>MTIKTKAELLNKWKPLLEGEGLPEIANSKQAIIAKIFENQEKDFQTAPEYKDEKIAQAFGSFLTEAEIGGDHGYNATNIAAGQTSGAVTQIGPAVMGMVRRAIPNLIAFDICGVQPMNSPTGQVFALRAVYGKDPVAAGAKEAFHPMYGPDAMFSGQGAAKKFPALAASTQTTVGDIYTHFFQETGTVYLQASVQVTIDAGATDAAKLDAEIKKQMEAGALVEIAEGMATSIAELQEGFNGSTDNPWNEMGFRIDKQVIEAKSRQLKAAYSIELAQDLRAVHGMDADAELSGILATEIMLEINREVVDWINYSAQVGKSGMTLTPGSKAGVFDFQDPIDIRGARWAGESFKALLFQIDKEAVEIARQTGRGEGNFIIASRNVVNVLASVDTGISYAAQGLATGFSTDTTKSVFAGVLGGKYRVYIDQYAKQDYFTVGYKGPNEMDAGIYYAPYVALTPLRGSDPKNFQPVMGFKTRYGIGINPFAESAAQAPASRIQSGMPSILNSLGKNAYFRRVYVKGI[186x];>[11x]MAKINELLRESTTTNSNSIGRPNLVALTRATTKLIYSDIVATQRTNQPVAAFYGIKYLNPDNEFTFKTGATYAGEAGYVDREQITELTEESKLTLNKGDLFKYNNIVYKVLEDTPFATIEESDLELALQIAIVLLKVRLFSDAASTSKFESSDSEIADARFQINKWQTAVKSRKLKTGITVELAQDLEANGFDAPNFLEDLLATEMADEINKDILQSLITVSKRYKVTGITDSGFIDLSYASAPEAGRSLYRMVCEMVSHIQKESTYTATFCVASARAAAILAASGWLKHKPEDDKYLSQNAYGFLANGLPLYCDTNSPLDYVIVGVVENIGEKEIVGSIFYAPYTEGLDLDDPEHVGAFKVVVDPESLQPSIGLLVRYALSANPYTVAKDEKEARIIDGGDMDKMAGRSDLSVLLGVKLPKIIIDE;>[172x]MASARGYVNIKTFEQKLDGNKKIEGKEVSVAFPLYSDV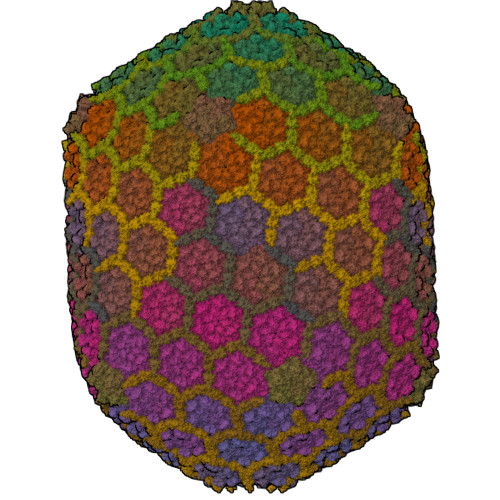HKISGAHYQTFPSEKAAYSTVYEENQRTEWIAANEDLWKVTG> MAKDELPIVNPEETGNLTDWDNEPTVSDLKSDYDSAYSSHSAQMSQITTWLNNLNVEGSAKPKKVPGRSSVQPMLIRKQAEWRYSALTEPFLSTDELFAVSPVTWEDREAAIQNQLVLNYQFNIKIDKVRFIDDYVRNAVNEGTVIVRVGWCNYTQMVKETVPVYAYYPAANEDQVAALQEALQLKLENPNAYNSLPDDIIASVDYSFENRGAFVAVQTGTEEVEYEKVIKNQPTVEVVNSQNVVIDPTCNGDISQAQFVIYSFETSKSDLEKDGRYKNLDKISASMSNPLNTPDHQVEDQSGFNFKDEPRKKFVAYEYWGWWDINGNGKTVPIVATFVGNTMIRLEENPFPDKKIPFVVVPYLPVPRSIYGEPDGALLEDNQKIIGATTRAMIDILARSANGQTGIRKDMLDVTNRRKFDKGEDYEFNANVDPRQGIYMHVSPEIPQSAPMMIQYQNNEAESLTGVKSFSQGIASQALGDVAAGIRGALDAASKRELGILRRLAQGVVEIGRKIISMNSEFLSEEEVVRVTNEQFVTVRRDELAGEFDLKLSISTAEADNQKAQELAFMLQTMGNSLPFEMSQMVLSDIARLRNMP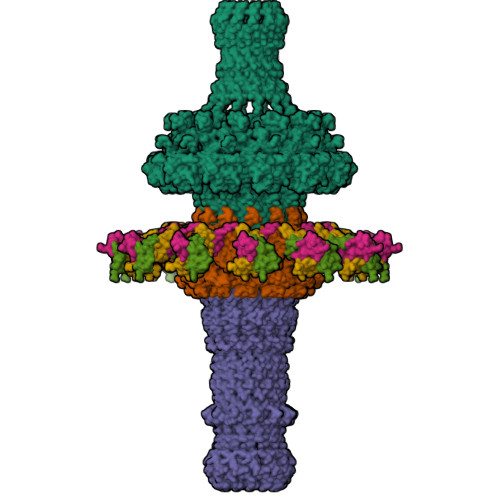DLAKRIESYQPQPDPLAQRKAELEIALLEAQIAETQSKAIENRASAGYKATQAQNVQSDTDLKNLDYVEQESGVKQARDVQKISAQAESQTQTKIVDYILKSGKPLSEI;> MKLSELFQMLSVGELSLIRTGNDGQGIRTQDYPKVIAQLNAGLTNLHARFPLLEKEVIIQQYEQISKYYLRSEFAQMNTTSTEKYKYLMDSPTERFLDDVIRVERVFDECGCPLYLNNEPCCGSIVTPSFDCIQIVYPIETNALFVTYRANHPKIALTTTDLNTEVRIPASHEKALTYYIASQLYSNSPNPETAAKGVEWSQRFEAECTKIENLDLDNAHIAQTNVKPEMRGWV;> MAVVIEPITNEDLTTKVVDGTGIFDELMTAANAHLSAQWDMERITGTQYAEVYLGQLTAVLQQAVTFLIEKDKTYLNNLLINAQIELANKQIELADKELEKADKEIELLELNKELIAQKVKTEKAQISDTVDSVPVTGIIGAQIALYKQQKDGFIRDAEQKALKIISDTWITRKTVDDGTPLPTGFDTAAVDAFTRKVADGVSVNY;>[3x]MIRTTNTCCGNQAGMVEKFIGTAYDVVKTVYDNLGEIQFIYNFLNDYGVLITVDSVTELQELPTTAKYTRVYSSTPTGVRIYTDYLYVEGDRTGVLPSDPTATGSWVVVGSSNSGAATGTGAYIPFVFNNGSAAGGETTIVVPDYTIGVPEIYVEGFRQQVGRGFTFNSVNLTVTLAQPLEQGDEVVLMLSGNPAVPDNPNIDSWTVINWIYNNGAAVGGEQVIVIPYTFQTVPAIFKNGLRYQGGLSTQSYTVDQDNKRILLTEPLSTNDRLVVQLGGELVTLESPDRSLYEIARATNMKDSEVIKSDNTVETLNGKRILYDIVSQVYYWIPSSVPNNVYIQSVVNGQLTYLPGNIVVTLTPIVTLGLSGTTAQRPIGVLTGTQHFDTTLGKPIWFNGTAWVDSTGAVV> MIELTSAPTTKIEIISAAISMVGKQQTVNTIDGGGALAIDAEKLYDTL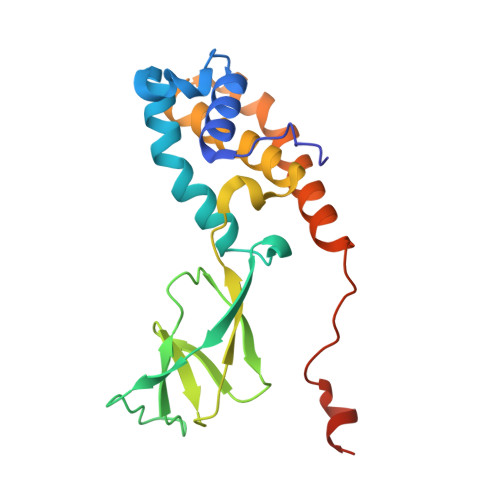VSAELGSNRWRFAQAFQQISIITTLNPTFDGWLYECQIPADCIMVQYLYPNIQYIVFGDKILTKSNQTFTLIYSRNVPVSKWPPPFSLYIVYHLASMLGISVTNSDRMLARISQGMEMWESRALFADAQSSVTLPFRHNPYVDVRYRYKTRGY(2R,3R,5R,6R)-5-acetamido-2,3-bis(fluoranyl)-6-[(1R,2R)-1,2,3-tris(oxidanyl)propyl]oxane-2-carboxylic 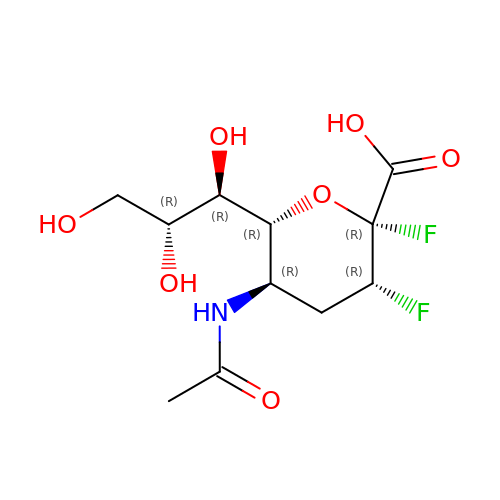acid | C11 H17 F2 N O7 | AHSNGFVNAWRJGS-WNBQUBFESA-N>[2x]GPLGSLANSVIDLIGNTPLVKINNIDTFGNEIYVKLEGSNPGRSTKDRIALKMIEEAEKEGLIDKDTVIIEATSGNTGIGLAMICAVKNYKLKIVMPDTMSIERIQLMRAYGTEVILTDGSLGMKACLEKLEELKKNEKKYFVPNQFT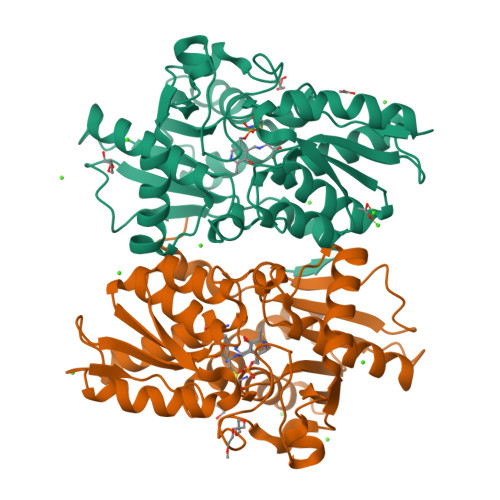NVNNPKAHYETTAEEILKDLNNKVDVFICGTGTGGSFSGTAKKLKEKLPNIKTFPVEPASSPLLSKGYIGPHKIQGMGMSIGGIPAVYDGSLADDILVCEDDDAFEMMRELSFKEGILGGISTGATFKAALDYSKENADKGLKIVVLSTDSGEKYLSNICDL> TYEEYGYDDTYAEQSYEGYEGYYSQSQGDS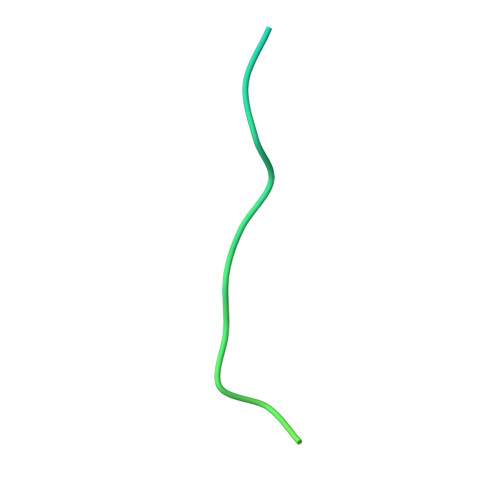EYYDYGHGEVQDSYEAYGQDDWNGT> MGSSHHHHHHSSGLVPRGSHMTTTISADQVNQIIYNLHHDPFEILGCHLLEEGKNTKKWVVRAYLPKAEAAWVIRPTERKEDPMNSVHHPNFFECIIETPELNHYQLKVKEGEHEKVIYDPYAFSSPYLTDEDIYLFSEGNHHRIYEKLGAHVGEINGVKGVYFAVWAPNARNVSVIGDFNNWDGREHQMRKRNYTIWELFVPEIGSGTVYKYEIKNSEGHIYEKSDPYGFYREVRPNTASIVVDIDNIYQWHDEEWLEKRRNSDPLKQPVSVYEVHLGSWLHGSSAEKMPLLNGEADPVIVSEWNPGARFLSYYELAEKLIPYVKDMGYTHIELLPIAEHPFDGSWGYQVTGFYSPTSRFGRPEDFMYFVDKCHENGIGVILDWVPGHFPKDSHGLAYFDGTHLYEHADPRIGEHKEWGTLVFNYGRHEVRNFLVANVLFW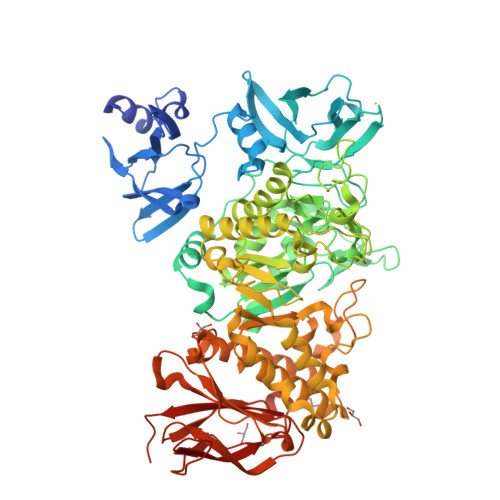FDKYHVDGIRVDAVASMLYRNYLRKEGEWIANEYGGDEHIEAVSFIREVNTLLFEYFPGILSIAEESTEWEKVSRPVYDGGLGFNLKWDMGWMHDMLDYFNIDPYFRQYHQNNVTFSMLYYYNENFMLALSHDEIVHGKSNMLGKMPGDEWQKYANVRALFTYMYTHPGKKTMFMSMEFGQWSEWNVAGDLEWHLLQYEPHQQLKQFFTDLNALYQQEPALYTHDFEYHGFEWIDCNDNTHSVVSFLRRSDDPNDSLVVVCNFTPQPHSHYRIGVPEAGYYVELFNSDAKQYGGSNMGNLGGKWADEWSFHNKPYSLDLCLPPLAVLILKLDPTKVPEGTTIKEIAADEEE> SSAHNAYNAGIMQKTGKAFADEFFAEENQVVH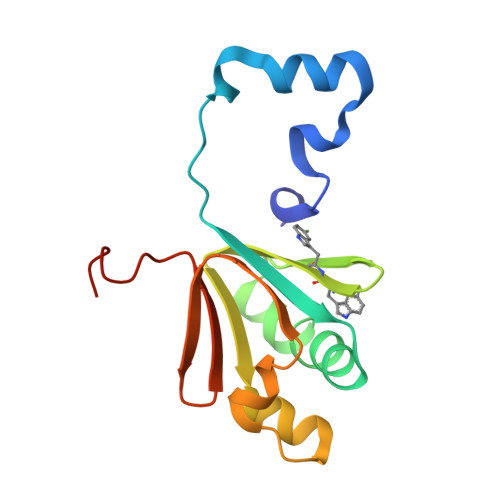ESNAVVLVLMKSDEIDAIIEDIVLKGGKAKNPSIVVEDKAGFWWIKADGAIEIDAAEAGELLGKPFSVYDLLINVSSTVGRAYTLGTKFTITSELMGLDRALTDI>GSAPIAKVTGPSTGAVGRNIEFSGKDSKDEDGKIVSYDWDFGDG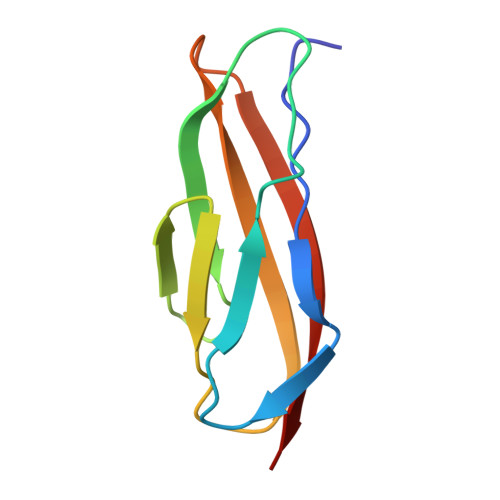ATSRGKNSVHAYKKAGTYNVTLKVTDDKGATATESFTIEIKNE[2x]>HMSKIYEDNSLTIGHTPLVRLNRIGNGRILAKVESRNPSFSVKCRIGANMIWDAEKRGVLKPGVELVEPTSGNTGIALAYVAAARGYKLTLTMPETMSIERRKLLKALGANLVLTEGAKGMKGAIQKAEEIVASDPQKYLLLQQFSNPANPEIHEKTTGPEIWEDTDGQVDVFISGVGTGGTLTGVTRYIKGTKGKTDLITVAVEPTDSPVIAQALAGEEIKPGPHKIQGIGAGFIPGNLDLKLIDKVVGITNEEAISTARRLMEEEGILAGISSGAAVAAALKLQEDESFTNKNIVVILPSSGERYLSTALFAD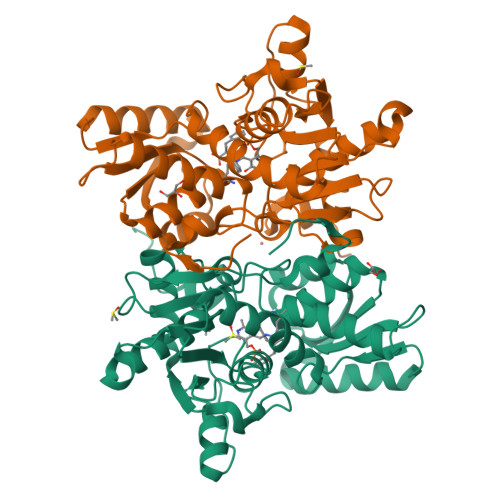LFTEKELQQ[2x]> MISPEQAMRERSELARKGIARAKSVVALAYAGGVLFVAENPSRSLQKISELYDRV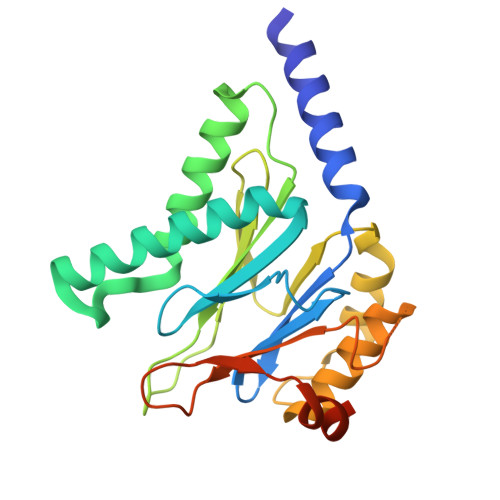GFAAAGKFNEFDNLRRGGIQFADTRGYAYDRRDVTGRQLANVYAQTLGTIFTEQAKPYEVELCVAEVAHYGETKRPELYRITYDGSIADEPHFVVMGGTTEPIANALKESYAENASLTDALRIAVAALRAGSADTSGGDQPTLGVASLEVAVLDANRPRRAFRRITGSALQALLVDQESPQSDGESSG>EEVRQFRRLFAQLAGDDMEVSATELMNILNKVVTRHPDLKTDGFGIDTCRSMVAVMDSDTTGKLGFEEFKYLWNNIKKWQAIYKQFDVDRSGTIGSSELPGAFEAAGFHLNEHLYSMIIRRYSDEGGNMDFDNFISCLV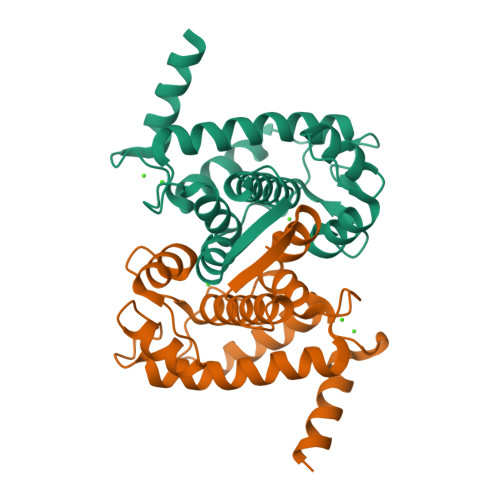RLDAMFRAFKSLDKDGTGQIQVNIQEWLQLTMYS[2x]> MSNGPEPHGNKIEQPEIRADERQDAGGPANGAPSTSGGAYSQGAKSGGQAAPD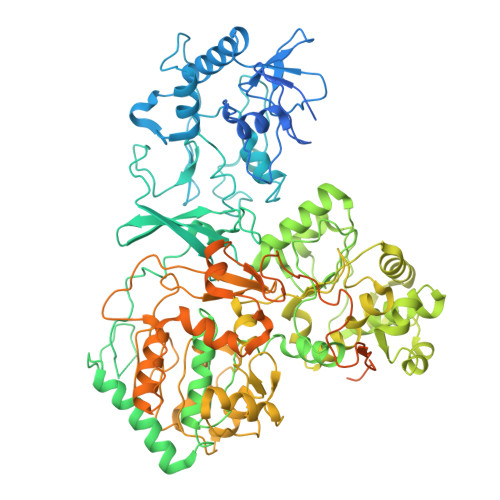PSGSYGIKDAPVAPATIAFEFDGQQVEAQPGETIWAVAKRLGTHIPHLCHKPDPGYRPDGNCRACMVEIEGERVLAASCKRTPAIGMKVKSATERATKARAMVLELLVADQPERATSHDPSSHFWVQADVLDVTESRFPAAERWTSDVSHPAMSVNLDACIQCNLCVRACREVQVNDVIGMAYRAAGSKVVFDFDDPMGGSTCVACGECVQACPTGALMPAAYLDANQTRTVYPDREVKSLCPYCGVGCQVSYKVKDERIVYAEGVNGPANQNRLCVKGRFGFDYVHHPHRLTVPLIRLENVPKDANDQVDPANPWTHFREATWEEALDRAAGGLKAIRDTNGRKALAGFGSAKGSNEEAYLFQKLVRLGFGTNNVDHCTRLCHASSVAALMEGLNSGAVTAPFSAALDAEVIVVIGANPTVNHPVAATFLKNAVKQRGAKLIIMDPRRQTLSRHAYRHLAFRPGSDVAMLNAMLNVIVTEGLYDEQYIAGYTENFEALREKIVDFTPEKMASVCGIDAETLREVARLYARAKSSLIFWGMGVSQHVHGTDNSRCLIALALITGQIGRPGTGLHPLRGQNNVQGASDAGLIPMVYPDYQSVEKDAVRELFEEFWGQSLDPQKGLTVVEIMRAIHAGEIRGMFVEGENPAMSDPDLNHARHALAMLDHLVVQDLFLTETAFHADVVLPASAFAEKAGTFTNTDRRVQIAQPVVAPPGDARQDWWIIQELARRLDLDWNYGGPADIFAEMAQVMPSLNNITWERLEREGAVTYPVDAPDQPGNEIIFYAGFPTESGRAKIVPAAIVPPDEVPDDEFPMVLSTGRVLEHWHTGSMTRRAGVLDALEPEAVAFMAPKELYRLGLRPGGSMRLETRRGAVVLKVRSDRDVPIGMIFMPFCYAEAAANLLTNPALDPLGKIPEFKFCAARVVPAEAAPMAAEHHHHHH>[4x]MSAPVTVKDLLSKPSAEIASFLGGIYEHSAWVAEALVKDAESLASIETISQLAAAMKAIVNKSSKDQKLELLCAHPDLCEKVGKLEMLTVESQEEQSRSGLQSLTDAELERFNSLNGAYRDQCGFPFILAVRNATKHTVLAALGGRVQHTPEQEFMVALEQVHKIAWMRLLSKIDTSDAQGFLTCHVLDTGNGCPAEKMRIHLHRLSPPEMAGLVGEFVTNDDGRL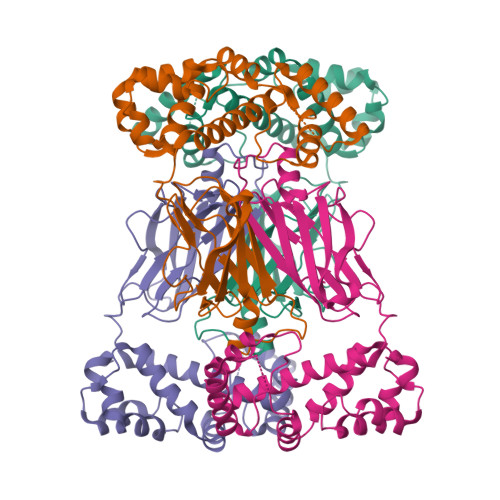EGGPALKGGKEFTVGQYEWTFFCGEYFASKGTFTSGQPFLDTIPLRFGIDNPDDHYHVPLLVSPWSFSTYRGS> GGCUUAUCAAGAGAGGGAGAGCGACUGGCGCGAAGAUCCCCGGCAACCAGAAAUGGUGCCAAUUCCUGCAGCGGAAACGUUGAAAGAUGAGCCG

One especially common junction element is the kink-turn (k-turn). k-turns are elements in double-stranded RNA that introduce a tight kink into the helical axis, with an included angle close to 50°. A standard k-turn comprises a three-nucleotide bulge followed by successive G•A and A•G trans G(sugar edge)•A(Hoogsteen edge) basepairs. k-turns are commonly-occurring motifs that introduce sharp kinks into duplex RNA, thereby facilitating tertiary contacts. Both the folding and conformation of k-turns are determined by their local sequence. k-turns fall into two conformational classes, called N3 and N1, that differ in the pattern of hydrogen bonding in the core. We show here that this is determined by the basepair adjacent to the critical G•A pairs.

We therefore decided to extend the study with a systematic structural analysis of HmKt-7 as a function of the 3b,3n sequence. This was performed in the constant environment of the SAM-I riboswitch, modified by replacing its natural k-turn by HmKt-7 with different 3b,3n sequences. In this way we could observe the effect of changing the 3b,3n sequence alone in an otherwise completely unchanged RNA molecule. Additionally, we hoped we might expand the range of 3b,3n sequences beyond the eight found in the natural k-turns to date. Six are completely new, i.e. 3b,3n = C•A, C–G, C•U, G•G, U–A and U•C, five of which adopt the N1 conformation. We note the majority (6/8) of the 3b = pyrimidine k-turns form N1 structures. Altogether seven of the new structures are in the N1 conformation, and clearly simply changing the 3b,3n sequence alone is sufficient to induce the structure of Kt-7 to change within the riboswitch environment. Evidently the 3b,3n sequence is the major determinant of the k-turn conformation.>MQWSGARALEALLTVAGELRGPPLQLDTGQLLKIAKRGGVTAVEAVHAWRNALTGAPLNLTPEQVVAIASHDGGKQALETVQRLLPVLCQAHGLTPQQVVAIASHDGGKQALETVQRLLPVLCQAHGLTPEQVVAIASHDGGKQALETVQALLPVLCQAHGLTPEQVVAIASNGGGKQALETVQRLLPVLCQAHGLTPQQVVAIASNGGGKQALETVQRLLPVLCQAHGLTPQQVVAIASNGGGKQALETVQRLLPVLCQAHGLTPQQVVAIASNCGGKQALETVQRLLPVLCQAHGLTPQQVVAIASNGGGKQALETVQRLLPVLCQAHGLTPQQVVAIASHDGGKQALETVQRLLPVLCQAHGLTPEQVVAIASNGGGKQALETVQRLLPVLCQAHGLTPEQVVAIASHDGGKQALETVQRLLPVLCQAHGLTPQQVVAIASNGGGRPALESIVAQLSRPDPALAALTNDHLVALACLGGRPALDAVKKLEHHHHHH[2x]

Transcription activator-like (TAL) effectors specifically bind to double stranded (ds) DNA through a central domain of tandem repeats. Each TAL effector (TALE) repeat comprises 33–35 amino acids and recognizes one specific DNA base through a highly variable residue at a fixed position in the repeat. The crystal structures of TAL effector (TALE) proteins bound to their respective target DNAs have revealed that the residue at position 13 is the only one directly involved in DNA base recognition, whereas the 12th residue stabilizes the proper loop conformation. dHax3, an engineered TALE protein, proved to be a useful scaffold for structural characterizations. We then present fifteen crystal structures of engineered dHax3 variants in complex with target DNA molecules, which elucidate the structural basis for the recognition of bases adenine (A) and guanine (G) by reported or uncharacterized TALE codes.

The structural observation suggests that Ile34 may not be a major contributor to the affinity of DNA binding by TALE repeats, consistent with the classification of NI as a “weak” TALE code. It also insinuates that base A may “tolerate” a wide range of amino acids at position 34 of a TALE repeat when there is no steric clash. To test this speculation, we generated dHax3 variants with the 34th residue on repeat 7 substituted with different amino acids. In total, we obtained nine high-quality structures that elucidate the accommodation of base A by Leu, Met, Cys, Pro, Trp, His, Thr, Asn, and Glu at the 34th position. Among these, the hydrophobic residues Leu, Met, Cys, and Pro all adopt conformations that do not clash with base A. As what happens to Ile34, there is no specific coordination found between these hydrophobic residues and base A. Trp, Thr, and His, in spite of the presence of polar groups, do not form H-bond with base A. They also appear to adopt conformations that simply avoid steric clash. These residues may all represent weak code, if they are used for base recognition.> MDEFEMIKRNTSEIISEEELREVLKKDEKSAHIGFEPSGKIHLGHYLQIKKMIDLQNAGFDII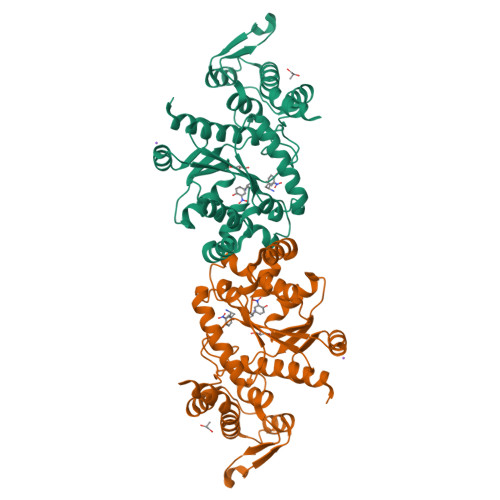ILLADLCAYLNQKGELDEIRKIGDYNKKVFEAMGLKAKYVYGSEFQLDKDYTLNVYRLALKTTLKRARRSMELIAREDENPKVAEVIYPIMQVNCAHYRGVDVAVGGMEQRKIHMLARELLPKKVVCIHNPVLTGLDGEGKMSSSKGNFIAVDDSPEEIRAKIKKAYCPAGVVEGNPIMEIAKYFLEYPLTIKRPEKFGGDLTVNSYEELESLFKNKELHPMDLKNAVAEELIKILEPIRKRLLEHHHHHH> QLWVDS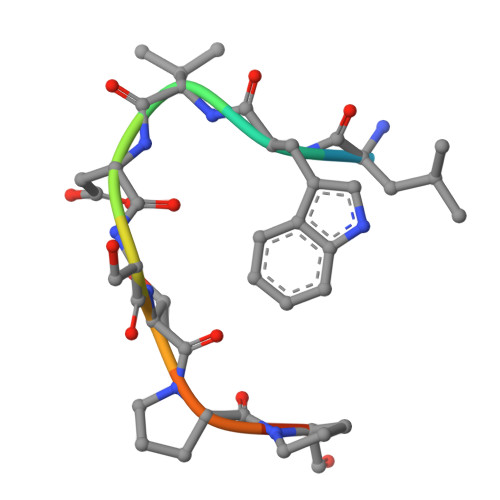TPPPG> MDWKKYGYNTRALHAGYEPPEQATGSRAVPIYQTTSYVFRDSDHAARLFALEEPGFIYTRIGNPTVSVLEERIAALEEGVGALAVASGQAAITYAILNIAGPGDEIVSGSALYGGTYNLFRHTLYKKSGIIVKFVDETDPKNIEEAITEKTKAVYLETIGNPGLTVPDFEAIAEIAHRHGVPLIVDNTVAPYIFRPFEHGADIVVYSATKFIGGHGTSIGGLIVDSGKFDWTNGKFPELVEPDPSYHGVSYVETFKEAAYIAKCRTQLLRDLGSCMSPFNAFLFILGLETLSLRMKKHCENALKIVEFLKSHPAVSWVNYP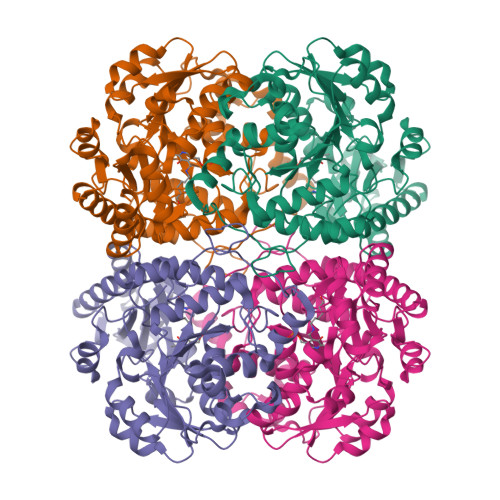IAEGNKTRENALKYLKEGYGAIVTFGVKGGKEAGKKFIDSLTLISHLANIGDARTLAIHPASTTHQQLTEEEQLKTGVTPDMIRLSVGIEDVEDIIADLDQALRKSQEG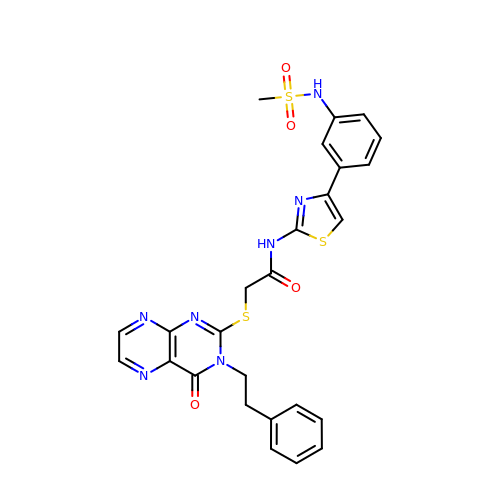~{N}-[4-[3-(methylsulfonylamino)phenyl]-1,3-thiazol-2-yl]-2-[4-oxidanylidene-3-(2-phenylethyl)pteridin-2-yl]sulfanyl-ethanamide | C26 H23 N7 O4 S3 | ZQUVBPXCXCKORU-UHFFFAOYSA-N> GGUAGACUCGCAGGAAGUCUACCGAGUAAGAGAAAGAGGAAAGACGGCCAAAUUGCGGGAAAGGGGACAACAGCCGUUCAGUACCAAGUCUCAGGGAAACUUCAGAUGGCCUCGCAAAGGGUAUGGUAAUAAGCUGACGGACAUGGUCCUAACCACGCAGUCAAGUCCUAAGUCAACAGCCUUGGCU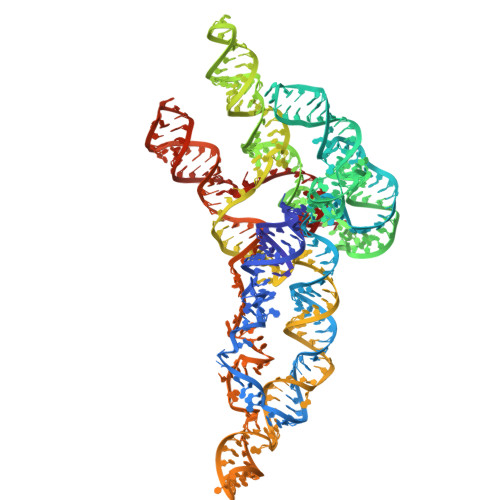GUUGAUAUGGAUGCAUUUCGAUCCAACCGAGGCUCAUUCUUGUAAUUCAUGGCCGUCGGGGAGGCACUUCGGUGCCUCUGAUAACAACUUGAAAUAAGGUUGGCUCAACGGCGCGUGACAGACAAUUCGCGCUGGAACUGCAGUCGGACCU> KES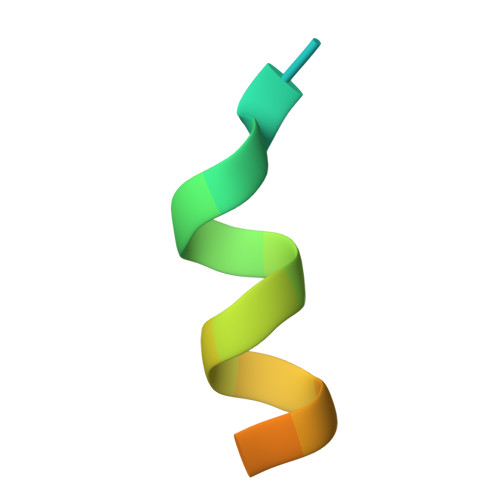KDHQLLRYLLDKDEKDLR> GPSTEDVPGDPQDVKATPLNSTSIHVSWKPPLEKDRNGIIRGYH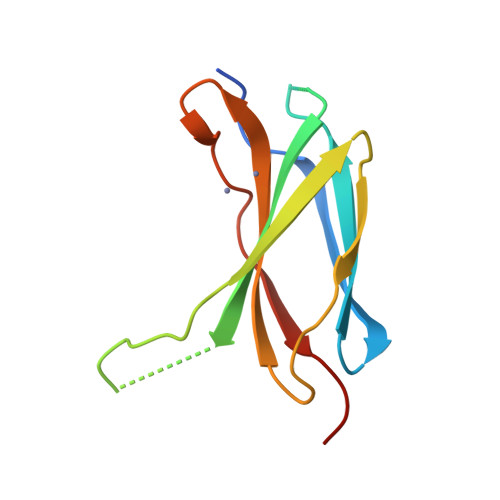IHAQELRDEGKGFLNEPFKFDVVDTLEFNVTGLQPDTKYSIQVAALTRKGDGDRSAAIVVKTPGGVP>MTATAETSTGTKVVLGQNQYGKAEVRLVKVTRNTARHEIQDLNVTSQLRGDFEAAHTAGDNAHVVATDTQKNTVYAFARDGFATTEEFLLRLGKHFTEGFDWVTGGRWAAQQFFWDRINDHDHAFSRNKSEVRTAVLEISGSEQAIVAGIEGLTVLKSTGSEFHGFPRDKYTTLQETTDRILATDVSARWRYNTVEVDFDAVYASVRGLLLKAFAETHSLALQQTMYEMGRAVIETHPEIDEIKMSLPNKHH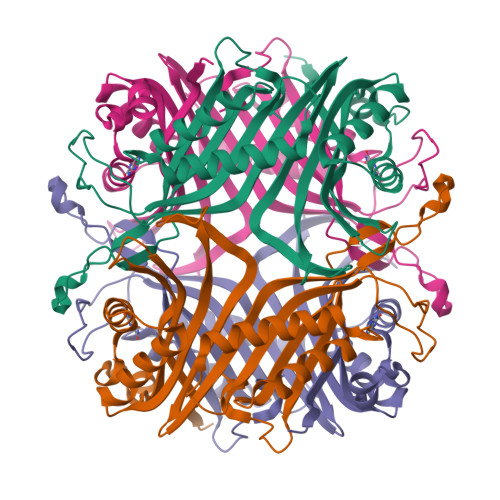FLVDLQPFGQDNPNEVFYAADRPYGLIEATIQREGSRADHPIWSNIAGFC[8x]> ASPISTIQPKANFDAQQFAGTWLLVAVGSAARFLQEQGHRAEATTLHVAPQGTAMAVSTFRKLDGICWQVRQLYGDTGVLGRFLLQARGARGAVHVVVAETDYQSFAVLYLE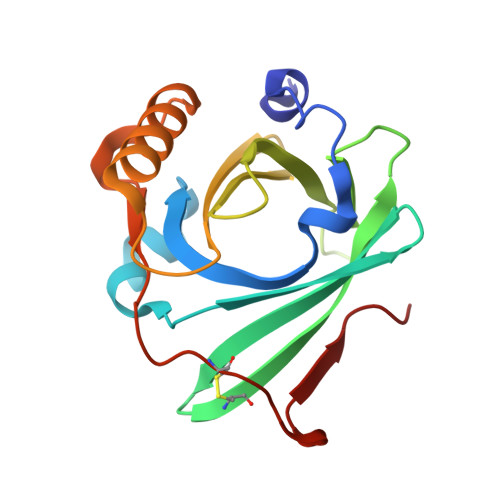RAGQLSVKLYARSLPVSDSVLSGFEQRVQEAHLTEDQIFYFPKYGFCEAADQFHVLDEVRR>[2x]MNRIAEAFEELKKKGEKALIPFITAGDPDLETTLELVRALVEAGADIIELGIPFSDPLADGPTIQRASQRALASGTTLDKVFEMVRELREKNTDVPIVFLTYYNPIFRYGIERFVKECAEAGVD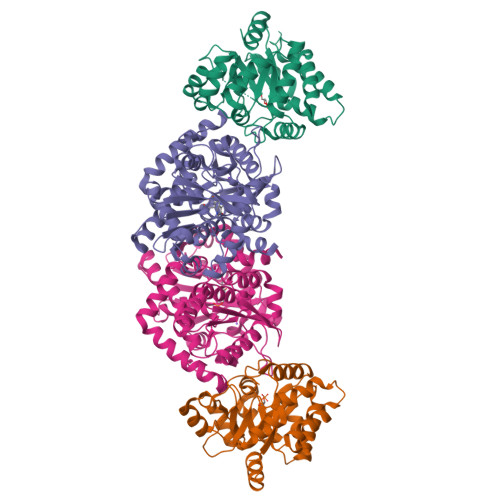GLIVPDLPPEEAADLAAAAEKYGVDLIFLVAPTSTDERIKMIAKHASGFVYCVSVTGVTGARSEIAADLAELVSRIRKHTDLPIAVGFGISTPEQAAEVAQVADGVIVGSAIVKRIEENQDEEDIVEEVREFVRELREAVKLEHHHHHH;>GRFGKYGGQYVPETLMPALEELEEAYERAKNDPEFQAELEYYLRDYVGRPTPLYFAENLTKDLGGAKIYLKREDLNHTGAHKINNALGQALLAKRMGKKRVIAETGAGQHGVATATVAAMFGLECVVYMGAEDIERQALNVFRMKLLGAKVRPVTSGSRTLKDAINEAMRDWVTNVEDTFYIIGSVVGPHPYPMMVRDFQSVIGEEARQQILEKEGRLPDAIVACVGGGSNAMGIFHPFIDDESVRLIGVEAAGKGIETGKHAATLSAGRPGVLHGAMTYLLQDEDGQIIEAHSISAGLDYPGVGPEHAYLKDTGRAEYVSVTDDEALEAFQLLSRTEGIIPALESSHAVAYAMKLAPELSKDQIIVVNLSGRGDKDVNTVARYLLGVELDLEHHHHHH[2x]6-{[2-(morpholin-4-yl)benzyl]amino}pyridine-3-carboxamide | C17 H20 N4 O2 | 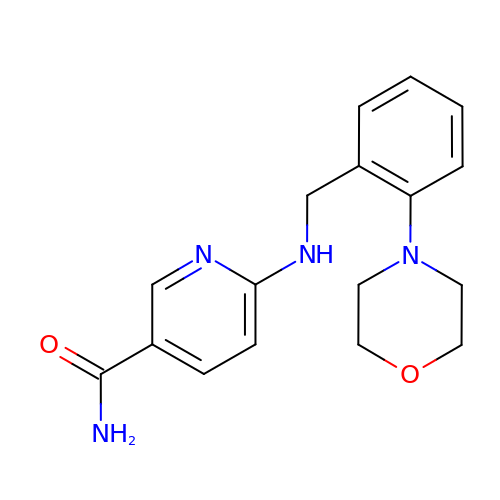OCZBFCMTTLGFND-UHFFFAOYSA-N(2~{S})-2-[[2-methyl-3-oxidanyl-5-(phosphonooxymethyl)pyridin-4-yl]methylamino]-4-oxidanyl-butanoic 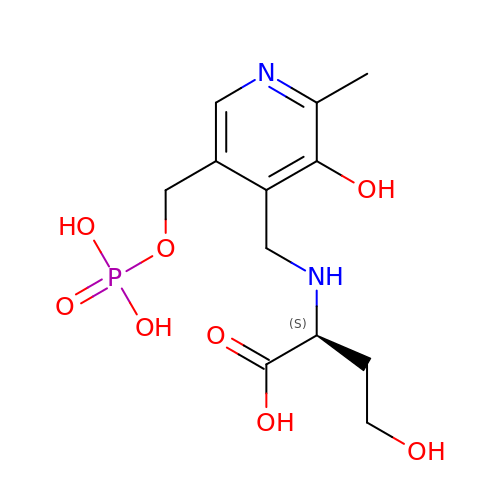acid | C12 H19 N2 O8 P | GLDZRPISEAFFFS-JTQLQIEISA-N>GSMDRKVAREFRHKVDFLIENDAEKDYLYDVLRMYHQTMDVAVLVGDLKLVINEPSRLPLFDAIRPLIPLKHQVEYDQLTPRRSRKLKEVRLDRLHPEGLGLSVRGGLEFGCGLFISHLIKGGQADSVGLQVGDEIVRINGYSISSCTHEEVINLIRTKKTVSIKVRHIGLIPVKSSPDEPLTWQYVDQFVSESGG[2x];>GSEEDAVDATPLEVFLQSQHLEEFLPIFMREQIDLEALLLCSDEDLQNIHMQLGPRKKV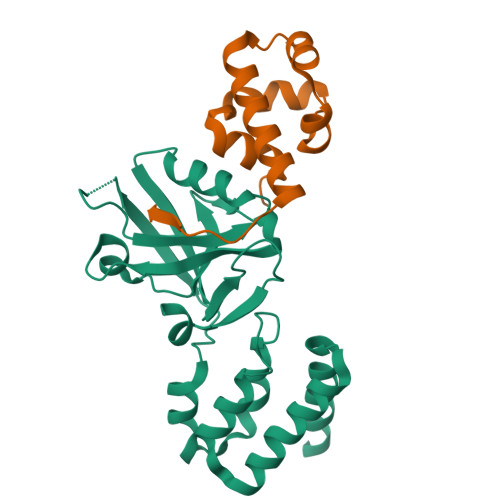LSAIDKRKQVLQQPGQLVDTSL[2x]> MDIISKSGEGNKYTINSAIAFVAYASHIDINTTEFSKVLSGLRDFINDEAIRLGGKISDGSFN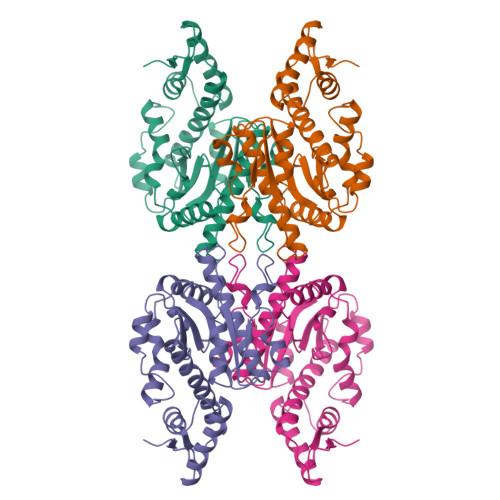KCNGDWYEWLIGIRAIEFFLESETNFIVVKMPNATSFDVMSIYKSCLSEFIYDLRSKLSLNNVNLITSNPDFSIIDIRGRREELKSMLKDISFSNISLSTISEIDNLYKNFIDYAELEHIKSFLSVKTTFRPDRRLQLAHEGSLMKALYTHLQTRTWTINPTGIRYYAAATSIGNADVIGLKTVATHSITDVKSLPQSAVDEIFKINSVLDVDSCLSHILSS TMEM106B is a type II transmembrane protein of 274 residues that localizes to late endosomes and lysosomes. Here we used structure determination by cryogenic electron microscopy to show that residues 120–254 of the lysosomal type II transmembrane protein 106B (TMEM106B) also form amyloid filaments in human brains. The TMEM106B folds shared a similar five-layered ordered core comprising residues S120–G254 and contained 17 β-strands, each ranging between 3 and 15 residues. We observed three TMEM106B folds, with no clear relationships between folds and diseases.

In fold II, these internal cavities are smaller than in fold I. We observed two subtypes of fold II (IIa and IIb) that differed mainly by the conformation of segment A167–I187. In folds IIb and III, there is a large extra density at the end of the side chain of K178, suggesting that this residue may be post-translationally modified. Fold II was found only in case 19, which was homozygous for T185. Although we did not solve the structures of filaments comprising two protofilaments of folds II or III, the micrographs of case 19, the only individual for which we observed filaments with fold IIa/b, and the micrographs of case 21, with fold III, also contained wider filaments that probably comprised two TMEM106B protofilaments. Our best maps for filaments with folds I, II and III had resolutions of 2.6, 3.4 and 2.8 Å, and came from case 1 (sporadic Alzheimer’s disease), case 19 (MSA) and case 17 (MSA), respectively. We divide the sequence that forms the ordered cores of the folds into three regions according to their degree of structural conservation: the amino-terminal region (S120–T166) is conserved in all three folds; the C-terminal region (Y211–G254) is conserved only in folds I and II; and the middle region (A167–M210) varies between folds.

>[3x]MGKSLSHLPLHSSKEDAYDGVTSENMRNGLVNSEVHNEDGRNGDVSQFPYVEFTGRDSVTCPTCQGTGRIPRGQENQLVALIPYSDQRLRPRRTKLYVMASVFVCLLLSGLAVFFLFPRSIDVKYIGVKSAYVSYDVQKRTIYLNITNTLNITNNNYYSVEVENITAQVQFSKTVIGKARLNNITIIGPLDMKQIDYTVPTVIAEEMSYMYDFCTLISIKVHNIVLMMQVTVTTTYFGHSEQISQERYQYVDCGRNTTYQLGQSEYLNVLQPQQ> NIKQFNNMIECTVPAR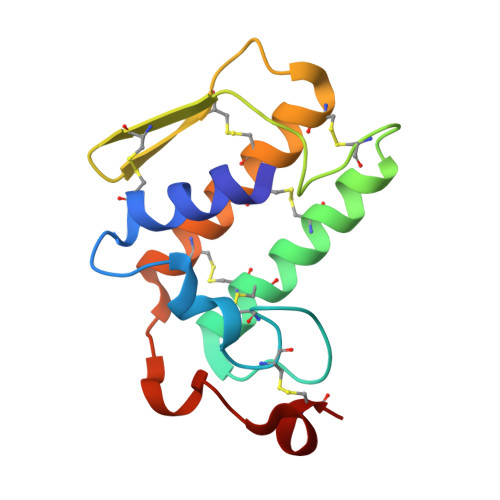SWWDFADYGCYCGSGSGSPTDDLDRCCQTHDNCYGAGGGSTGCAPKSRTYTYQCSQGTLTCSGENSACAATTCDCDRLAAICFAGAPYNDTNYNIDLKSRCQ>MYQAGGTIRSLLDKVAEQEYLLPAIQREFVWRPEQICRLFDSLLQGYPFGTFLFWKIKPENRDSYQFYQFMQHYHERDNYHCENVTQLPEREFIAVLDGQQRITALNIGLRGSFAWKLTGKWWSNDDAFPVRRLHLNLLSKPDLETGSMYDFEFLTDDKASLDASEQYWFRVGRIMEEEEDALIDEVADDARLSSEQRKEARSTLRHLYRTIHDKDKISFYEESDQSLERVLNIFIRMNSGGTTLSYSDLLLSIAVAQWSSLDAREEIHALVDEMNRVGDGFNVSKDLVLKAGLMLSDIGSVGFKVENFNKENMAILEKNWTPIRDALLLSMQLLASFGFNAQNLRATSAILPLAYYLHHRKLTASYLSRVEYAVDRECIRNWLIRSLLKASGIWGSGLDTLLTMLRSDIKQSGDTGFPLAKIEATMQQRGKSLRFDPEEISELAQLDYGNPRTFALLTLLFPGFDFSRHFHVDHIYPKGLFTRNKLAKVGVPAEQLDELIEASNKLPNLQ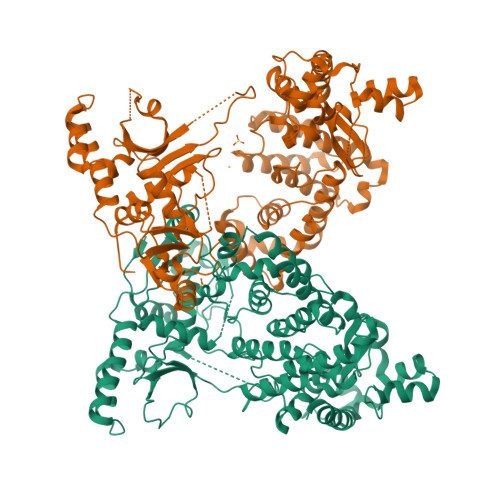LLEGTINNQKRQKMPHEWYAQQWPDVNARQAHLQSQAITSLPEQLNQFMDFYRERQETLLARIRTALQPASSVETE[2x]>[3x]MMEVFMNFLDQLDLIIQN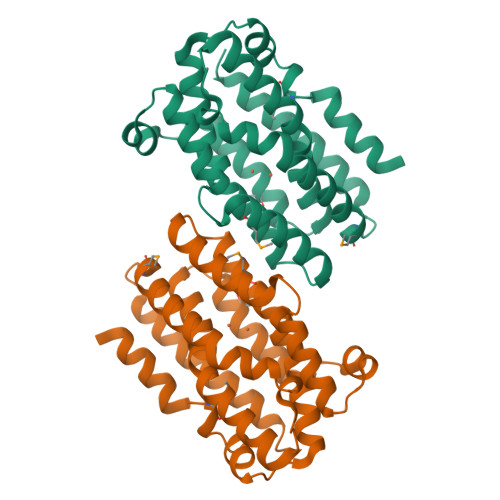KHMLEHTFYVKWSKGELTKEQLQAYAKDYYLHIKAFPKYLSAIHSRCDDLEARKLLLDNLMDEENGYPNHIDLWKQFVFALGVTPEELEAHEPSEAAKAKVATFMRWCTGDSLAAGVAALYSYESQIPRIAREKIRGLTEYFGFSNPEDYAYFTEHEEADVRHAREEKALIEMLLKDDADKVLEASQEVTQSLYGFLDSFLDPGTCCSCHQSY> UG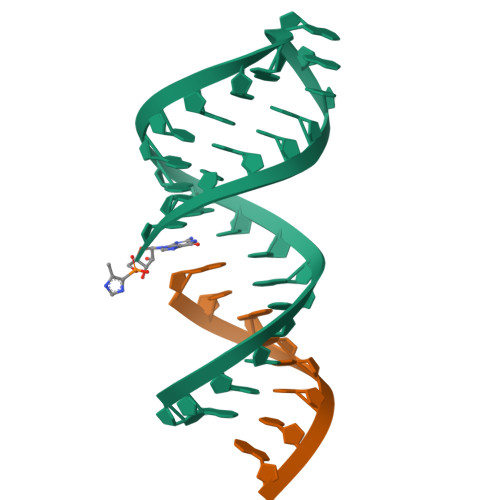AGGUGNNGAGCGCGAAAGCGCUC;> GCACCUCA The ethylene-forming enzyme (EFE) is an Fe(II), 2-oxoglutarate (2OG), and l-arginine (l-Arg)-dependent oxygenase that either forms ethylene and three CO2/bicarbonate from 2OG or couples the decarboxylation of 2OG to C5 hydroxylation of l-Arg. l-Arg binds with C5 toward the metal center, causing 2OG to change from monodentate to chelate metal interaction and OD1 to OD2 switch of D191 metal coordination. The best characterized EFE is that from the Pseudomonas savastanoi (formerly Pseudomonas syringae) pv phaseolicola strain PK2, for which several crystal structures have been reported. This enzyme binds mononuclear Fe(II) using three side chains (H189, D191, and H268) with three water molecules completing the six-coordinate geometry. Here, we extend our understanding of EFE catalysis by carrying out biochemical, structural, and computational studies of the enzyme in complex with a substrate analogue and using two enzyme variants. In combination, the results presented here are compatible with the currently proposed enzyme mechanism,4−8 emphasize the necessity for OD2 of D191 to coordinate the metal, and highlight the importance of the second coordination sphere and longer range interactions in promoting EFE activity.

Second, we examined the R171A variant of the EFE,9 a substitution of a second-sphere residue (i.e., just beyond the immediate metal ligands) that eliminates ethylene-forming activity likely by destabilizing 2OG binding. We carried out MLCT analysis and elucidated the R171A EFE crystal structure to provide evidence for significant changes in the 2OG binding pocket that explain the abolishment of activity, and we used electrospray ionization–mass spectrometry (ESI-MS) to identify an unanticipated ligand at the 2OG binding site. Alanine substitution of R171, a residue that forms a hydrogen bond with the C1 carboxylate of 2OG, leads to a significant shift of the loop containing residues 80–94, a loss in activity, and an inability to form the chromophore associated with chelate binding of Fe(II) by 2OG. These changes cause reduced stability of binding 2OG, leading to the adventitious binding of benzoate at the 2OG binding site. The source of benzoate is unclear, analogous to the situation for crystals of canavalin, a jack bean vicilin protein, that was purified from E. coli cells and shown to have bound benzoate. The R171A EFE had electron density at the 2OG binding site that was identified by mass spectrometry as benzoic acid. Substituting alanine for R171 that interacts with 2OG and l-Arg inactivates the protein, prevents metal chelation by 2OG, and weakens l-Arg binding.

> MTNLQTFELPTEVTGCAADISLGRALIQAWQKDGIFQIKTDSEQDRKTQEAMAASKQFCKEPLTFKSSCVSDLTYSGYVASGEEVTAGKPDFPEIFTVCKDLSVGDQRVKAGWPCHGPVPWPNNTYQKSMKTFMEELGLAGERLLKLTALGFELPINTFTDLTRDGWHHMAVLRFPPQTSTLSRGIGAHTDYGLLVIAAQDDVGGLYIRPPVEGEKRNRNWLPGESSAGMFEHDEPWTFVTPTPGVWTVFPGDILQFMTGGQLLSTPHKVKLNTRERFACAYFHEPNFEASAYPLFEPSANERIHYGEHFTNMFMRCYPDRITTQRINKENRLAHLEDLKKYSDTRATGS> MDEFEMIKRNTSEIISEEELREVLKKDEKSAEIGFEPSGKIHLGHYLQIKKMIDLQNAGFDIIISLAD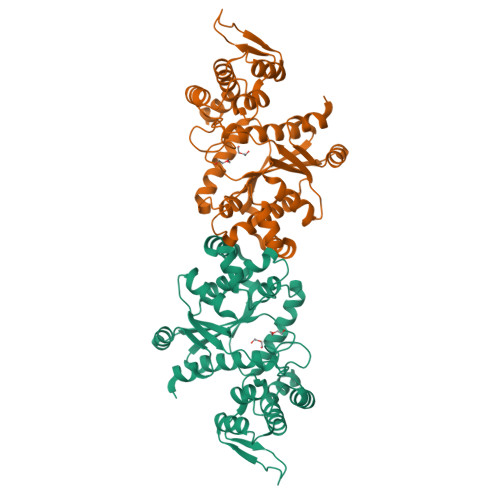LGAYLNQKGELDEIRKIGDYNKKVFEAMGLKAKYVYGSEFGLDKDYTLNVYRLALKTTLKRARRSMELIAREDENPKVAEVIYPIMQVNNIHYVGVDVAVGGMEQRKIHMLARELLPKKVVCIHNPVLTGLDGEGKMSSSKGNFIAVDDSPEEIRAKIKKAYCPAGVVEGNPIMEIAKYFLEYPLTIKRPEKFGGDLTVNSYEELESLFKNKELHPMDLKNAVAEELIKILEPIRKRLAHHHHH>MAEARSQPSAGPQLNALPDHSPLLQPGLAALRRRAREAGVPLAPLPLTDSFLLRFLRARDFDLDLAWRLLKNYYKWRAECPEISADLHPRSIIGLLKAGYHGVLRSRDPTGSKVLIYRIAHWDPKVFTAYDVFRVSLITSELIVQEVETQRNGIKAIFDLEGWQFSHAFQITPSVAKKIAAVLTDSFPLKVRGIHLINEPVIFHAVFSMIKPFLTEKIKERIHMHGNNYKQSLLQHFPDILPLEYGGEEFSMEDICQE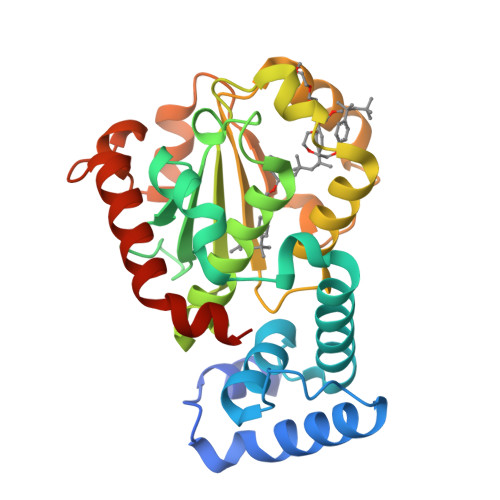WTNFIMKSEDYLSSISESIQ[2x]> MGGSSHHHHHHSSGLVPRGSGGLTHRKFGGSGGSPFSGLSSIAVRSGSWLDAIIIDGVHHGGSGGNLSPTFTFGSGEYISNMTIRSGDWIDNISFETNMGRRFGPYGGSGG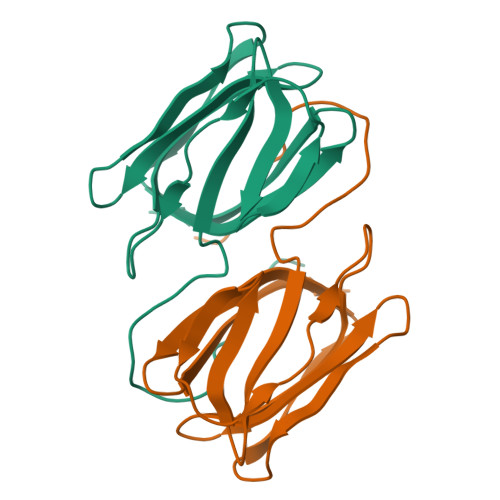SANTLSNVKVIQINGSAGDWLDSLDIYYEQY>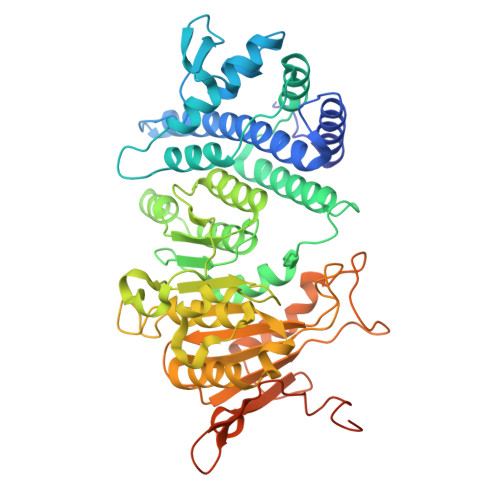 MTIRFMARTKKADQPMTTAQQLGAIVKSSRQIMRKDKGLNGDLDRLPMLTWIMFLKFLDDLEQMRETEAVLEGKSFQPAIEAPYRWRDWAAIEGGITGDELIAFINNDEAMRPDGTRGIGLFAYLRSLQGDNGGDRRDVIATVFKGMQNRMINGYLLRDVVDKINGIHFNSSEEMHTLSRLYETMLREMRDAAGDSGEFYTPRPVVRFMVEVMDPQLGESVLDPACGTGGFLVEAFEHLERQCKTVEDREVLQESSIFGGEAKSLPYLLVQMNLLLHGLEYPRIDPENSLRFPLREMGDKDRVDVILTNPPFGGEEEKGILGNFPEDMQTAETAMLFLQLIMRKLKRPGHGSDNGGRAAVVVPNGTLFSDGISARIKEELLKNFNLHTIVRLPEGVFAPYTDIAGNLLFFDRSGPTDDIWYYQITVPEGRKKYTKTKPMESHEFDECLNWWSNRIVNQNAWKESASEIIKYSESGQLIDVNLDRKNPNSLEVLEHEEPMDLIEKITTKEESLLAILEQIKAEISTQGISK>[2x]MKTIIINGVQFNTDEDTTILKFARDNNIDISALCFLNNCNNDINKCEICTVEVEGTGLVTACDTLIEDGMIINTNSDAVNEKIKSRISQLLDIHEFKCGPCNRRENCEFLKLVIKYKARASKPFLPKDKTEYVDERSKSLTVDRTKCLLCGRCVNACGKNTETYAMKFLNKNGKTIIGAEDEKCFDDTNCLLCGQCIIACPVAALSEKSHMDRVKNALNAPEKHVIVAMAPSVRASIGELFNMGFGVDVTGKIYTALRQLGFDKIFDINFGADMTIMEEATALVQRIENNGPFPMFTSCCPGWVRQAENYYPELLNNLSSAKSPQQIFGTASKTYYPSISGLDPKNVFTVTVMPCTSKKFEADRPQMEKDGLRDIDAVITTRELAKMIKDAKIPFAKLEDSEADPAMGEYSGAGAIFGATGGVMEAALRSAKDFAENAELEDIEYKQVRGLNGIKEAEVEINNNKYNVAVINGASNLFKFMKSGMINEKQYHFIEVMACHGGCVN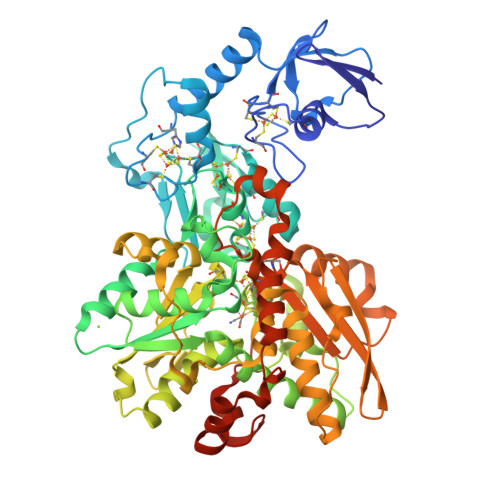GGGQPHVNPKDLEKVDIKKVRASVLYNQDEHLSKRKSHENTALVKMYQNYFGKPGEGRAHEILHFKYKKSAWSHPQFEK>[2x]MGHHHHHHMPMYEVQWKVGEESNGNNYSYIDPTQLPYDHKWEFPRNRLSFGKTLGAGAFGKVVEATAQGLIKSDAAMTVAVKMLKPSAHSTEREALMSELKVLSYLGNHENIVNLLGACTHGGPTLVITEYCCYGDL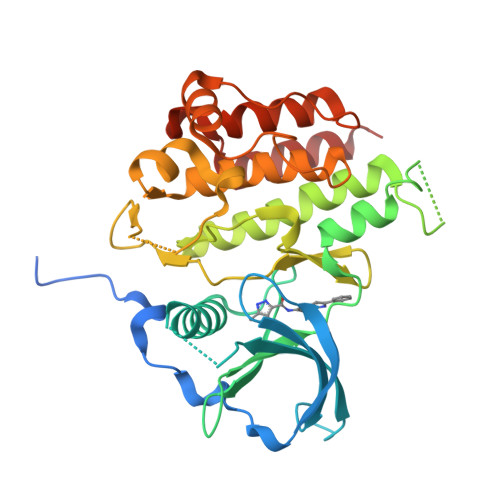LNFLRRKRDSFHSSDTSPASMEDDENALDLEDLLSFSYQVAKGMAFLASKNCIHRDLAARNILLTHGRITKICDFGLARVIKNDSNYVDKGNARLPVKWMAPESIFNSVYTFESDVWSYGIFLWELFSLGSSPYPGMPVDSKFYKMIKEGFRMSSPEHAPAEMYDIMKTCWDADPDKRPTFKQIVQDIEKQISESTNH>MPKPYVAINMAELKNEPKTFEMFASVGPKVCMVTARHPGFVGFQNHIQIGILPFGNRYGGAKMDMTKESSTVRVLQYTFWKDWKDHEEMHRQNWSYLFRLCYSCASQMIWGPWE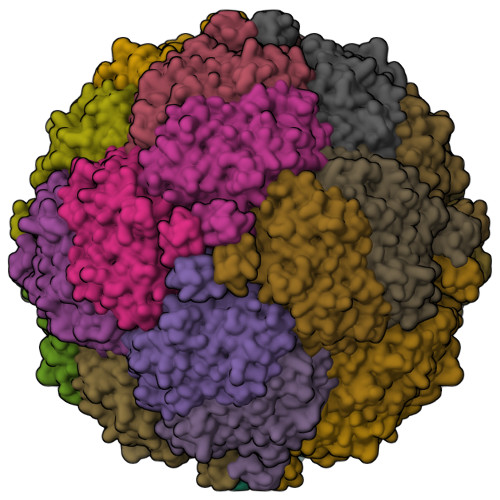PIYEIIYANMPINTEMTDFTAVVGKKFAEGKPLDIPVISQPYGKRVVAFAEHSVIPGKEKQFEDAIVRTLEMLKKAPGFLGAMVLKEIGVSGIGSMQFGAKGFHQVLENPGSLEPDPNNVMYSVPEAKNTPQQYIVHVEWANTDALMFGMGRVLLYPELRQVHDEVLDTLVYGPYIRILNPMMEGTFWREYLNENAWRHPQFGG[6x]> XXXXXXXXXXXXXXXXXXXXXXXXXXXXXXXXXXXXXXXXSQNLEEEKKQRNHFKSIQAKILEKYGTHKPESPVLKIVNVTQTSCVLAWDPLKLGSAKLKSLILYRKGIRSMVIPNPFKVTTTKISGLSVDTPYEFQLKLITTSGTLWSEKVILRTHKMTDMSGITVCLGPLDPLKEISDLQISQCLSHIGARPLQRHVAIDTTHFVCNDLDNEESNEELIRAKHNNIPIVRPEWVRACEVEKRIVGVRGFYLDADQSILKSYTFPPVNEEELSYSKENEPVAEVADENK;> MNLFWPSETKKQNEIPGGDYTPGNSPSVQKGYQFLNRDIFKSCPRIMERQFGECLHNRTHLIKDLISSGNVGLGPIEIVHMSYLNKHEKEEFGEYFYVTGIEVSGPAMPVEFLEVLKSSKRISKNISNNIILTYCCFNFFSNLDIRIRYDADDTFQTTAIDCNKETTDLTMTEKMWEETFASSVIRAIITNTNPELKPPGLVECPFYVGKDTISSCKKIIELLCRFLPRSLNCGWDSTKSMQATIVNNYLMYSLKSFIAITPSLVDFTIDYLKGLTKKDPIHDIYYKTAMITILDHIETKELDMITILNETLDPLLSLLNDLPPRDADSARLMNCMSDLLNIQ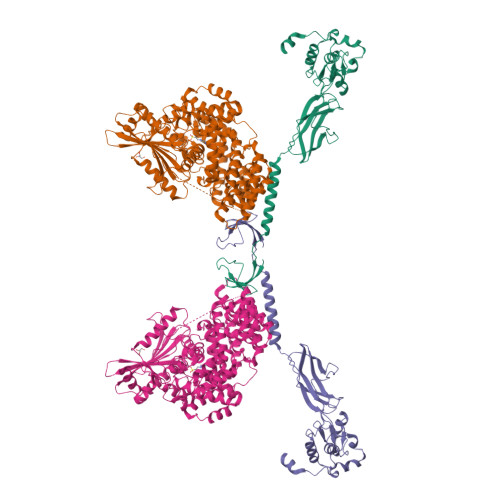TNFLLNRGDYELALGVSNTSTELALDSFESWYNLARCHIKKEEYEKALFAINSMPRLRKNDGHLETMYSRFLTSNYYKKPLNGTREHYDLTAMEFTNLSGTLRNWKEDELKRQIFGRIAMINEKKIGYTKEIWDDIAIKLGPICGPQSVNLINYVSPQEVKNIKNINLIARNTIGKQLGWFSGKIYGLLMEIVNKIGWNGLLNIRTEAFMMETEFYQASNNIIDENGHIPMESRKKRFCEGWLDDLFLDLYQDLKLSKISLSNKDEKHSGLEWELLGLIMLRTWHWEDAVACLRTSIVARFDPVSCQQLLKIYLQPPKNIQEVTLLDTDTIISLLIKKISYDCRYYNYCQIFNLQLLEKLCNELGTHILRNKILLQPSIGDEIMVMIDAMLAWIADLDHTVQPGTENLYFQ> GNNEYKKGLWTVEEDKILMD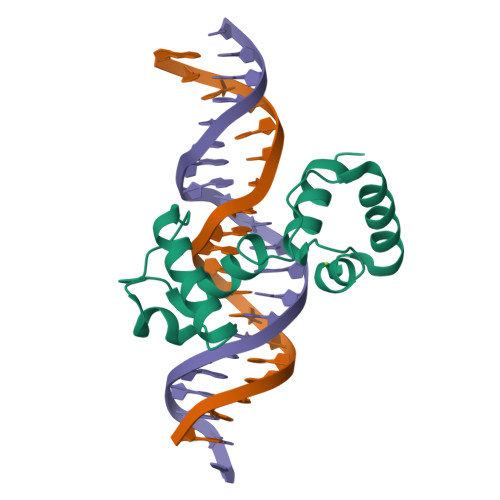YVKAHGKGHWNRIAKKTGLKRCGKSCRLRWMNYLSPNVKRGNFTEQEEDLIIRLHKLLGNRWSLIAKRVPGRTDNQVKNYWNTHLSKKLGIKDQKTKQS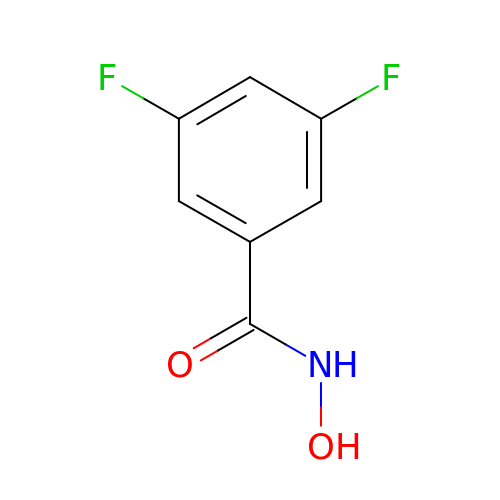3,5-difluoro-N-hydroxybenzamide | C7 H5 F2 N O2 | HIJCVQNNEDULLG-UHFFFAOYSA-N> AGSVDTVSLYSGRGANMPFTIMEAESTSNATNGTKLTPNFKPGDYAGEASGRSSVYLDATGEYVEFTLTSPANAFVLRNAVAENTTGTVSIYADGVSKGKFNVSSKFSYLYATPSTLGRLGYDNAPGAGLTAYWLYED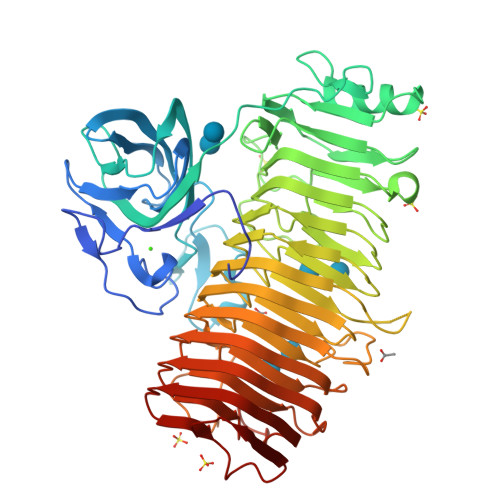AQLMLDQVYPAGTKIKIQKDAGDVSWIYVDLLETENVAPPQANPDPTKYVAVSASKSIDQALTEFRQDNTKKGIYIPAGEWTINSKIFLYGRATEIVGAGPWYTKLVAPQSQSNTDVGFNISAAANGSTIRDLSAWGNYINRVDGPGKFIDGNGMQNVTVQNIWVEHFVCLYWGVNSSYNTFKNNRIKNTFAAGINMTNGSSYNVIDNNYARGTGDDSFALFSATDSGGSYNVGNKYTNLTATNVRRAAAFAVYGGSDNLFQNLYGADTLTYPGITISSYSFGYNTLGFGDQDTVIDGATLDRTGGDFWTSVGADDKINEYQNFGAIWIYGGDRAIKNILIKNVDINNPVYFGLMFQSMSPNNMVMQNIRVENVNINNPSRYGIKLVVRAEQGQGPAYGGASFTNVKVNNPGISAIYGEAQSPNFTVTRVSGNNW> SMGGPQYGIAREDVVLNRILGEGFFGEVYEGVY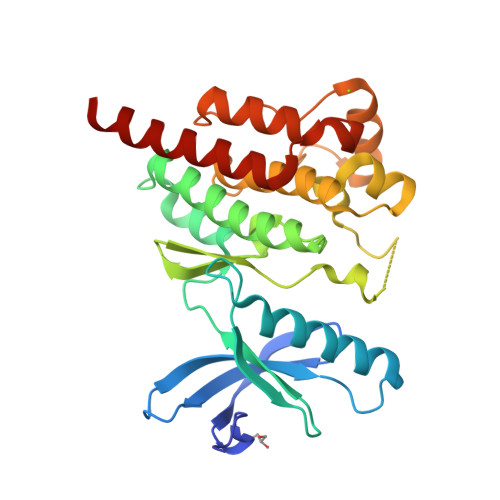TNHKGEKINVAVKTCKKDCTLDNKEKFMSEAVIMKNLDHPHIVKLIGIIEEEPTWIIMELYPYGELGHYLERNKNSLKVLTLVLYSLQICKAMAYLESINCVHRDIAVRNILVASPECVKLGDFGLSRYIEDEDYYKASVTRLPIKWMSPESINFRRFTTASDVWMFAVCMWEILSFGKQPFFWLENKDVIGVLEKGDRLPKPDLCPPVLYTLMTRCWDYDPSDRPRFTELVCSLSDVYQMEKDIAME> TDTAEAVPKFEEMFA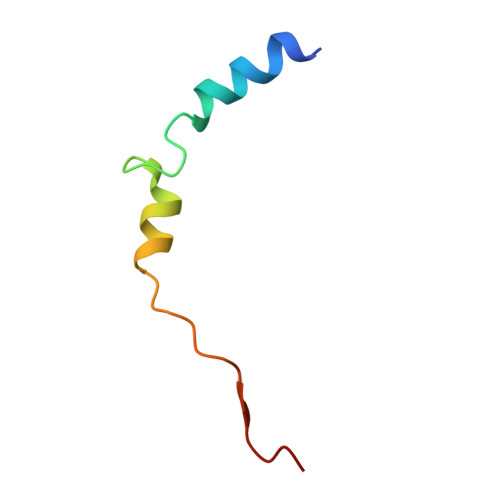SRFTENDKEYQEYLKRPPESPPIVEEWNS> MDKEIYCGSVPVSYFDPFDLFESLRPEFQQILPLDNIHWKAFDGTVRTVNRLPIELIPEGRGEADKSNDEQPFIRFLIVNCISIDQYRAKVRPLVRQWLPNLESVSSSTGEKMIYKPIILLYANSEVVDSNLFKSVSLMEKFGKDFPHVQTLEVRSVYRSPKERQEFWNQFSQKIKASVLSIFQKRLTHLQHSLANLQKGNNFEEQLLTREKLYELYVVFNILEDASLELQKIKKEILRRNMNMPDGKLQVPFESSSKSDESLGSIIIEGTLDKFQLHKYFFIRRLRLLKLEDQTLTAFVGAFQLIKNFIESISIEYRKSVRLLEFKHYFITSMLSYFEFENVSNPLLCEIKAELLMLKRDNWVQGVMATSGYRLMDKNYPNSDVKYKFDLLKETFVDETVFQENFLTLTKEILSLFNKCEGKRQRIVDILSIEIGLLYYQGKKYEEAVSLFLSCYEYYTQTNWNSIGLKILQVFIDSLSHCPKLDVLQIDGESVSASAVLTNAFLNILKLCKDNDSKEIWWKKFMDLQMKNNIHLMYPLDGLFEVTLNSKV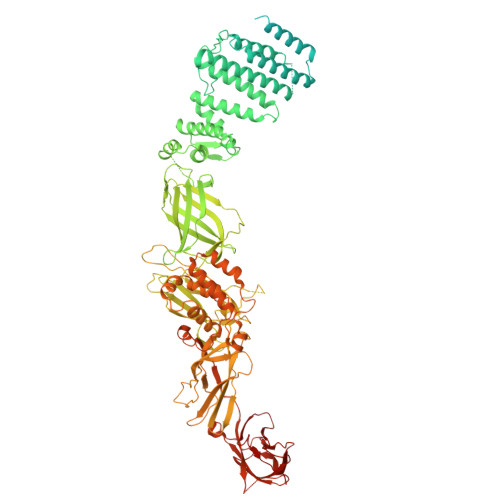HLARANVSAIEVNLKSYGFPEDISTKTMRLSLKNMGGDVIVFGASDFLLKKGENKLILECRDIMYGEFSLLSFEIIVEGITFVKEFPENQDEFIVVPEIYCKESTKVLVKQAHNLNLGEYALELKSVQSDALESLQVEVEVQKNIGNMKNLPVSFSMDEIQARKRYNTPFENVRLEYYLLDQITAFDLIIKTSFTKKNDQGTFGETKKVRIQCYLQLSVSVEDIFKKDIFFFKFLLNSSVREEPVILYSSELSAPDTRNDYNIRGDYIATTPALITFDGNESFINCYEITANNNFDSKDIFNLKVRYNTLKEQLDCFITDAVLIEGDVEWFILFEKWKTFWELEILKKLKYDYDAFKENRIIRLLKTSIDLNKTKSKIRNLCIEKAVLDKILICLNKVSRGIAVCNTDMDEYVRNLVPKQLTVPVQLPGFEQFFHVQFEQMETSHDALHDTIATIGNSLSYTVIVENLSGQWGQDVIDDGGYIFEILSSNEWLIHGQKRCAIKEKRKEFEVHLIPLKKGYLNFPRVEITNINGKSCRVDHSNAFESILIFAA ADENOSINE -5'-THIO-MONOPHOSPHATE | C10 H14 N5 O6 P S | 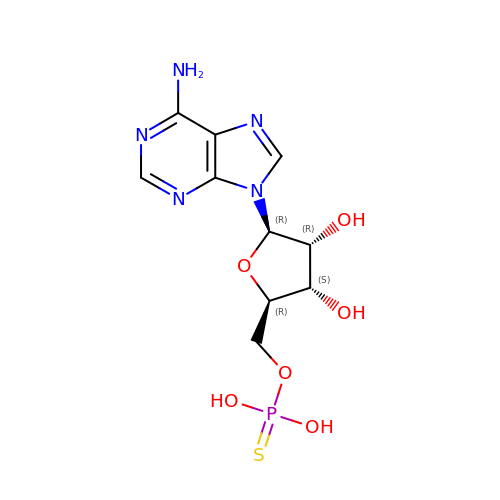UBCPYVAQZGCDJO-KQYNXXCUSA-N>MAHHHHHHMTIRVMLQAMDQGHLLVNNVDKYVRAGRGVMVYIAFLSDRDSAPITDEALRHAVGVLLHTKIFTHFSPEKMINQPQSLEECPEMDILIVPQASLGGKVKGRSVQFHQLVAKDVGAALYDRFCHFVRVARGVDESRVDANGAPRSEGDAPKAEGWIKYNSRVISGTFGNRQGLRFESEGPFTH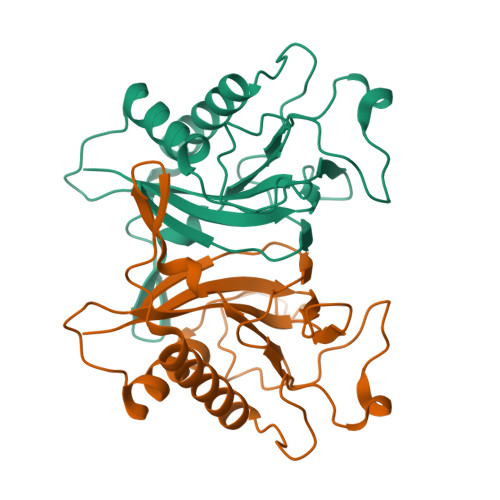MFDI[4x]>MGCGIMKYGITEMVKTIDTKTRVVDVTNEIAKKKYQAIRDFLEGEEFKEVVIFGVYLWGNYTAQMLSKYADKVYLVDIHEFMKGFVPNNNSIKFLNLNEFKLKFIRGEVNPDLIVDLTGLGGIEPEFLAKFNPKVFIV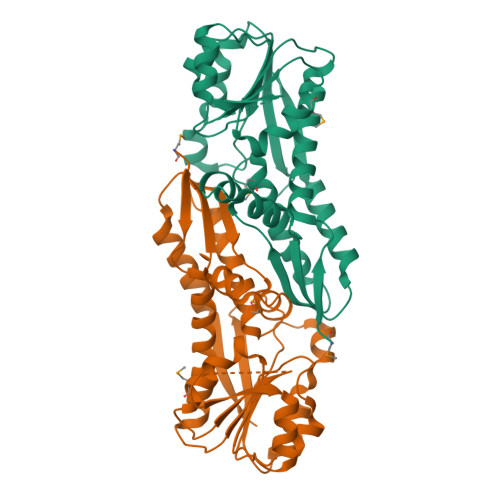EDPKGVFDVDIYEADNTYKRTAPFIEKAKVGVLKTYRKARVSKTSGTMTLTIDTIVDASREITSLDGVLYAIPNLRYYEGILFHENDIHKFLSEISQPAITISTLNDVLDEAEEILSNNINLIYSFVEEL[8x]> MPSKPLRPCNKIGCTN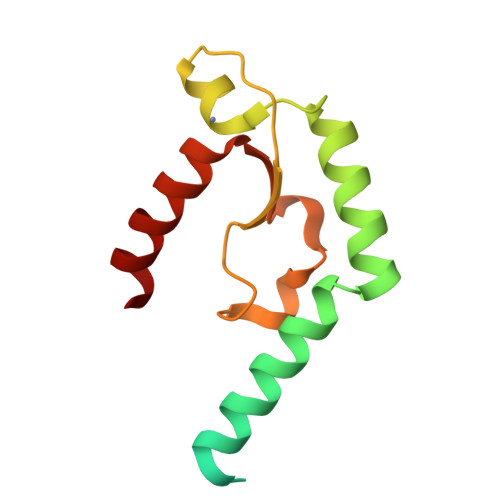LTRDRYCEQHKHLAEQRQRTRRNDKEYDKHKRNQQARAFYHSREWERTRLAVLAKDNYLCQHCLKEKKITRAVIVDHITPLLVDWSKRLDMDNLQSLCQACHNRKTAEDKRRYG>[2x]MGGSSHHHHHHSSGLVPRGSHMKLITASSSKEYLPDLLLFWQNYEYWITNIGLYKTKQRDLTRTPANLDTDTEECMFWMNYLQKDQSFQLMNFAMENLGALYFGSIGDISELYLRVEQYWDRRADKNHSVDGKYWDALIWSVFTMCIYYMPVEKLAEIFSVYPLHEYLGSNKRLNWEDGMQLVMCQNFARCSLFQLKQCDFMAHPDIRLVQAYLILATTTFPYDEPLLANSLLTQCIHTFKNFHVDDFRPLLNDDPVESIAKVTLGRIFYRLCGCDYLQSGPRKPIALHTEVSSLLQHAAYLQDLPNVDVYREENSTEVLYWKIISLDRDLDQYLNKSSKPPLKTLDAIRRELDIFQYKVDSLEEDFRSNNSRFQKFIALFQISTVSWKLFKMYLIYYDTADSLLKVIHYSKVIISLIVNNFHAKSEFFNRHPMVMQTITRVVSFISFYQIFVESAAVKQLLVDLTELTANLPTIFGSKLDKLVYLTERLSKLKLLWDKVQLLDSGDSFYHPVFKILQNDIKIIELKNDEMFSLIKGLGSLVPLNKLRQESLLEEEDENNTEPSDFRTIVEEFQSEYNISDILS;> MGVTSNVVLVSGEGERFTVDKKIAERSLLLKNYLNDMHDSNLQNNSDSESDSDSETNHKSKDNNNGDDDDEDDDEIVMPVPNVRSSVLQKVIEWAEHHRDSNFPDEDDDDSRKSAPVDSWDREFLKVDQEMLYEIILAANYLNIKPLLDAGCKVVAEMIRGRSPEEIRRTFNIVNDFTPEEEAAIRRENEWAEDRGS;> MGPSFNPVRFLELPIDIRKEVYFHLDGNFCGAHPYPIDILYKSNDVELPGKPSYKRSKRSKKLLRYMYPVFATYLNIFEYSPQLIEKWLEYAFWLRYDCLVLDCFKV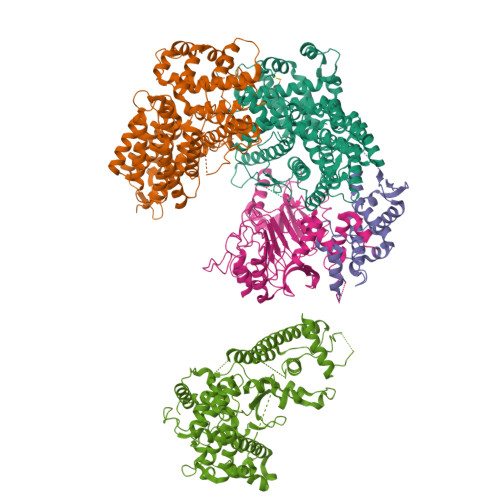NHLYDGTLIDALEWTYLDNELRLAYFNKASMLEVWYTFKEYKKWVIDSVAFDELDLLNVSNIQFNIDNLTPQLVDKCLSILEQKDLFATIGEVQFGQDEEVGEEKDVDVSGANSDENSSPSSTIKNKKRSASKRSHSDNGNVGATHNQLTSISVIRTIRSMESMKSLRKITVRGEKLYELLINFHGFRDNPGKTISYIVKRRINEIRLSRMNQISRTGLADFTRWDNLQKLVLSRVAYIDLNSIVFPKNFKSLTMKRVSKIKWWNIEENILKELKVDKRTFKSLYIKEDDSKFTKFFNLRHTRIKELDKSEINQITYLRCQAIVWLSFRTLNHIKLQNVSEVFNNIIVPRALFDSKRVEIYRCEKISQVLVIGSRSGSENLYFQGSKRRWKKNFIAVSAANRFKKISSSGAL;> MGRSSILFLLKLMKIMDVQQQQEAMSSEDRFQELVDSLKPRTAHQYKTYYTKYIQWCQLNQIIPTPEDNSVNSVPYKDLPISAELIHWFLLDTLITDDKPGEKREETEDLDEEEENSFKIATLKKIIGSLNFLSKLCKVHENPNANIDTKYLESVTKLHTHWIDSQKAITTNETNNTNTQVLCPPLLKVSLNLWNPETNHLSEKFFKTCSEKLRFLVDFQLRSYLNLSFEERSKIRFGSLKLGKRDRDAIIYHKVTHSAEKKDTPGHHQLLALLPQDCPFICPQTTLAAYLYLRFYGIPSVSKGDGFPNLNADENGSLLQDIPILRGKSLTTYPREETFSNYYTTVFRYCHLPYKRREYFNKCNLVYPTWDEDTFRTFFNEENHGNWLEQPEAFAFPDKIPFDFKKIMNFKSPYTSYSTNAKKDPFPPPKDLLVQIFPEIDEYKRHDYEGLSQNSRDFLDLMEVLRERFLSNLPWIYKFFPNHDIFQDPIFGNSDFQSYFNDKTIHSKGSPILSFDILPGFNKIYKNKTNFYSLLIERPSQLTFASSHNPDTHPWSHPQFEK>MVKAIESYDEWKTLTSGSDVVVVDYWATWCGPCKMISPHFAKLEGKFPNVKFAKVDVEEQEDIAKEAQIKAMPTFVAYKDGKVI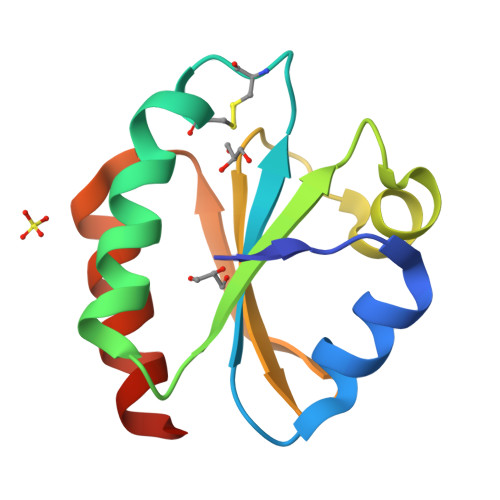ETVTGAVPAKINALLDKVAAHHHHHH[2x]(2R)-2-[(1S)-1-methoxy-2-oxidanyl-2-oxidanylidene-ethyl]-5-methylidene-2H-1,3-thiazine-4-carboxylic acid | C9 H11 N O5 S | 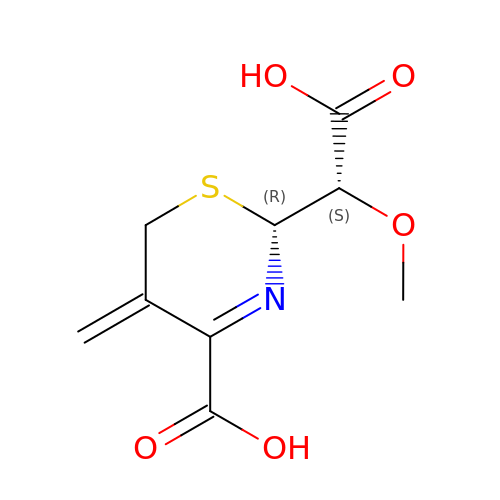DOPBSRLSQLUMSV-RNFRBKRXSA-N2-(6-{[(3-chloro-2-methylphenyl)sulfonyl]amino}pyridin-2-yl)-N,N-diethylacetamide | C18 H22 Cl N3 O3 S | 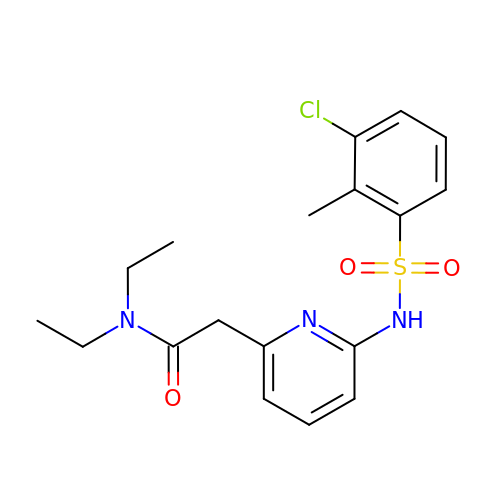JNWQLOFSMUGRNY-UHFFFAOYSA-N> TLKLCSPEEFTRLCREKTQEIYPIKEANGRTRKALIICNTEFKHLSLRYGANFDIIGMKGLLEDLGYDVVVKEELTAEGMESEMKDFAALSEHQTSDSTFLVLMSHGTLHGICGTMHSEKTPDVLQYD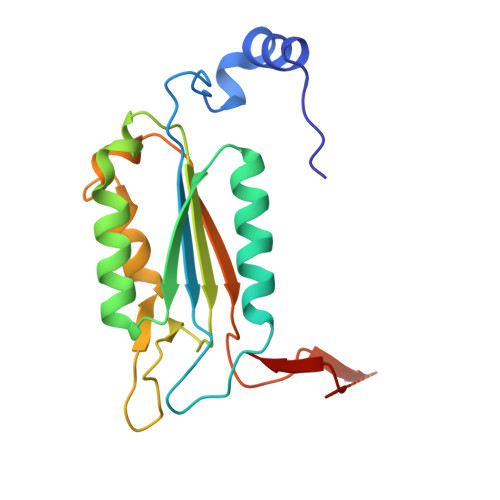TIYQIFNNCHCPGLRDKPKVIIVQAARGGNSGEMWIRESSKPQLCRGVDLPRNMEAD2-(3,4-dichlorobenzyl)-5,6-dihydroxypyrimidine-4-carboxylic acid | C12 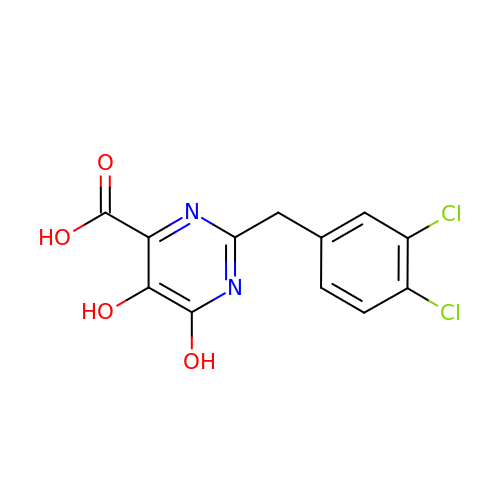H8 Cl2 N2 O4 | OZDSTVKQUHMIRA-UHFFFAOYSA-N>GSHMATYYYALASQKFLLEEEPFEEVLKERRRDYGEKNKEIDFWQVIQPAFLNAPELAEAKAKAPEKNVAIVSTNKSFIVWVKLALEYVLTGEFEAPSDAIPDPLASLD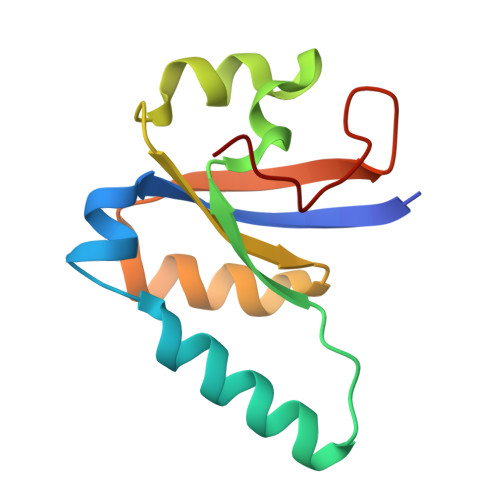[4x]5-{5-[(piperidin-4-yl)oxy]-2H-isoindol-2-yl}-4-(trifluoromethyl)pyridazin-3(2H)-one 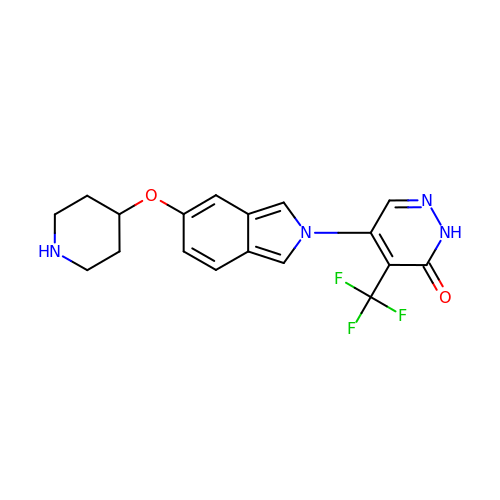| C18 H17 F3 N4 O2 | DPAMCOKMVSYBNR-UHFFFAOYSA-N> GPGSMRRVVVTGMGIVSSIGSNTEEVTASLREAKSGISRAEEYAELGFRCQVHGAPDIDIESLVDRRAMRFHGRGTAWNHIAMDQAIADAGLTEEEVSNERTGIIMGSGGPSTRTIVDSADITREKGPKRVGPFAVPKAMSSTASATLATFFKIKGINYSISSA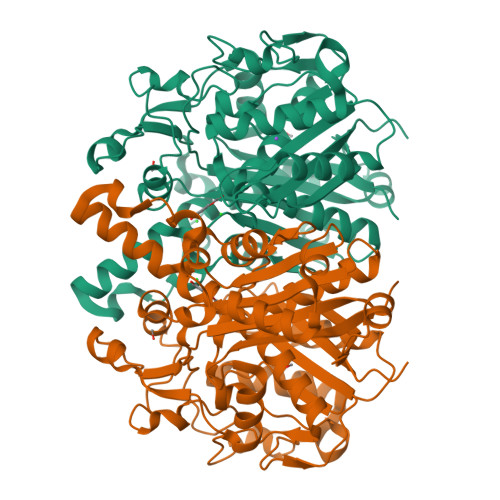CATSNHCIGNAYEMIQYGKQDRMFAGGCEDLDWTLSVLFDAMGAMSSKYNDTPSTASRAYDKNRDGFVIAGGAGVLVLEDLETALARGAKIYGEIVGYGATSDGYDMVAPSGEGAIRCMKMALSTVTSKIDYINPHATSTPAGDAPEIEAIRQIFGAGDVCPPIAATKSLTGHSLGATGVQEAIYSLLMMQNNFICESAHIEELDPAFADMPIVRKRIDNVQLNTVLSNSFGFGGTNATLVFQRYQG> MKIFSESHKTVFVVDHCPYMAESCRQHVEFDMLVKNRTQGIIPLAPISKSLWTCSVESSMEYCRIMYDIFPFKKLVNFIVSDSGAHVLNSWTQEDQNLQELMAALAAVGPPNPRADPECCSILHGLVAAVETLCKITEYQHEARTLLMENAERVGNRGRIICITNAKSDSHVRMLEDCVQETIHEHNKLAANSDHLMQIQKCELVLIHTYPVGEDSLVSDRSKKELSPVLTSEVHSVRAGRHLATKLNILVQQHFDLASTTITNIPMKEEQHANTSANYDVELLHHKDAHVDFLKSGDSHLGGGSREGSFKETITLKWCTPRTNNIELHYCTGAYRISPVDVNSRPSSCLTNFLLNGRSVLLEQPRKSGSKVISHMLSSHGGEIFLHVLSSSRSILEDPPSISEGCGGRVTDYRITDFGEFMRENRLTPFLDPRYKIDGSLEVPLERAKDQLEKHTRYWPMIISQTTIFNMQAVVPLASVIVKESLTEEDVLNCQKTIYNLVDMERKNDPLPISTVGTRGKGPKRDEQYRIMWNELETLVRAHINNSEKHQRVLECLMACRSKPPEEEERKKRGRKREDKEDKSEKAVKDYEQEKSWQDSERLKGILERGKEELAEAEIIKDSPDSPEPPNKKPLVEMDETPQVEKSKGPVSLLSLWSNRINTANSRKHQEFAGRLNSVNNRAELYQHLKEENGMETTENGKASRQ;> MPTVVVMDVSLSMTRPVSIEGSEEYQRKHLAAHGLTMLFEHMATNYKLEFTALVVFSSLWELMVPFTRDYNTLQEALSNMDDYDKTCLESALVGVCNIVQQEWGGAIPCQVVLVTDGCLGIGRGSLRHSLATQNQRSESNRFPLPFPFPSKLYIMCMANLEELQSTDSLECLERLIDLNNGEGQIFTIDGPLCLKNVQSMFGKLIDLAYTPFHAVLKCGHLTADVQVFPRPEPFVVDEEIDPIPKVINTDLEIVGFIDIADISSPPVLSRHLVLPIALNKEGDEVGTGITDDNEDENSANQIAGKIPNFCVLLHGSLKVEGMVAIVQLGPEWHGMLYSQADSKKKSNLMMSLFEPGPEPLPWLGKMAQLGPISDAKENPYGEDDNKSPFPLQPKNKRSYAQNVTVWIKPSGLQTDVQKILRNARKLPEKTQTFYKELNRLRKAALAFGFLDLLKGVADMLERECTLLPETAHPDAAFQLTHAAQQLKLASTGTSEYAAYDQNITPLHTDFSGSSTERI;> MSDIRHSLLRRDALSAAKEVLYHLDIYFSSQLQSAPLPIVDKGPVELLEEFVFQVPKERSAQPKRLNSLQELQLLEIMCNYFQEQTKDSVRQIIFSSLFSPQGNKADDSRMSLLGKLVSMAVAVCRIPVLECAASWLQRTPVVYCVRLAKALVDDYCCLVPGSIQTLKQIFSASPRFCCQFITSVTALYDLSSDDLIPPMDLLEMIVTWIFEDPRLILITFLNTPIAANLPIGFLELTPLVGLIRWCVKAPLAYKRKKKPPLSNGHVSNKVTKDPGVGMDRDSHLLYSKLHLSVLQVLMTLQLHLTEKNLYGRLGLILFDHMVPLVEEINRLADELNPLNASQEIELSLDRLAQALQVAMASGALLCTRDDLRTLCSRLPHNNLLQLVISGPVQQSPHAALPPGFYPHIHTPPLGYGAVPAHPAAHPALPTHPGHTFISGVTFPFRPIR;> MSAQGDCEFLVQRARELVPQDLWAAKAWLITARSLYPADFNIQYEMYTIERNAERTATAGRLLYDMFVNFPDQPVVWREISIITSALRNDSQDKQTQFLRSLFETLPGRVQCEMLLKVTEQCFNTLERSEMLLLLLRRFPETVVQHGVGLGEALLEAETIEEQESPVNCFRKLFVCDVLPLIINNHDVRLPANLLYKYLNKAAEFYINYVTRSTQIENQHQGAQDTSDLMSPSKRSSQKYIIEGLTEKSSQIVDPWERLFKILNVVGMRCEWQMDKGRRSYGDILHRMKDLCRYMNNFDSEAHAKYKNQVVYSTMLVFFKNAFQYVNSIQPSLFQGPNAPSQVPLVLLEDVSNVYGDVEIDRNKHIHKKRKLAEGRE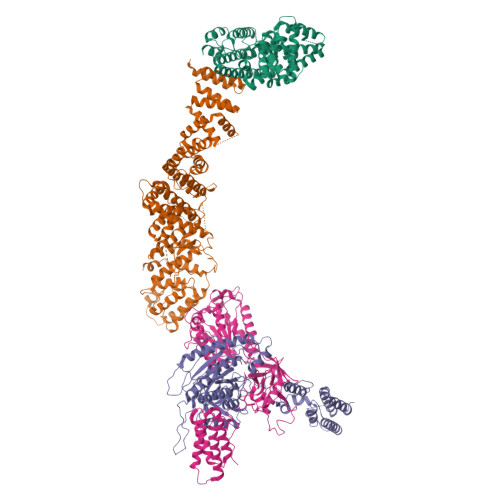KTMSSDDEDCSAKGRNRHIVVNKAELANSTEVLESFKLARESWELLYSLEFLDKEFTRICLAWKTDTWLWLRIFLTDMIIYQGQYKKAIASLHHLAALQGSISQPQITGQGTLEHQRALIQLATCHFALGEYRMTCEKVLDLMCYMVLPIQDGGKSQEEPSKVKPKFRKGSDLKLLPCTSKAIMPYCLHLMLACFKLRAFTDNRDDMALGHVIVLLQQEWPRGENLFLKAVNKICQQGNFQYENFFNYVTNIDMLEEFAYLRTQEGGKIHLELLPNQGMLIKHHTVTRGITKGVKEDFRLAMERQVSRCGENLMVVLHRFCINEKILLLQTLT>[3x]GPHMLEMKIFSESHKTVFVVDHCPYMAESCRQHSKSLWTCSVES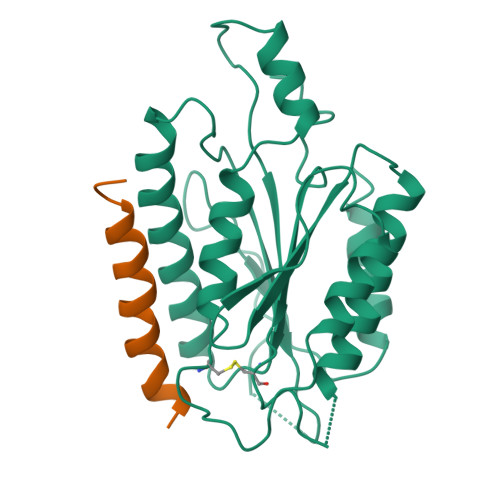SMEYCRIMYDIFPFKKLVNFIVSDSGAHVLNSWTQEDQNLQELMAALAAVGPPNPRADPECCSILHGLVAAVETLCKITEYQHEARTLLMENAERVGNRGRIICITNAKSDSHVRMLEDCVQETIHEHNKLAANSDHLMQIQKCELVLIHTYPVGEDSLVSDRSKKELSPVLTSEVHSVRAGRHLATKLNILVQQHFD;>[3x]GHMEDRLERLQEILRKFLYLEREFRQITIS>MSSDADAHKVGLIPVTLMVSGNIMGSGVFLLPANLASTGGIAIYGWLVTIIGALGLSMVYAKMSFLDPSPGGSYAYARRCFGPFLGYQTNVLYWLACWIGNIAMVVIGVGYLSYFFPILKDPLVLTITCVVVLWIFVLLNIVGPKMITRVQAVATVLALIPIVGIAVFGWFWFRGETYMAAWNVSGLGTFGAIQSTLNVTLWSFIGVESASVAAGVVKNPKRNVPIATIGGVLIAAVCYVLSTTAIMGMIPNAALRVSASPFGDAARMALGDTAGA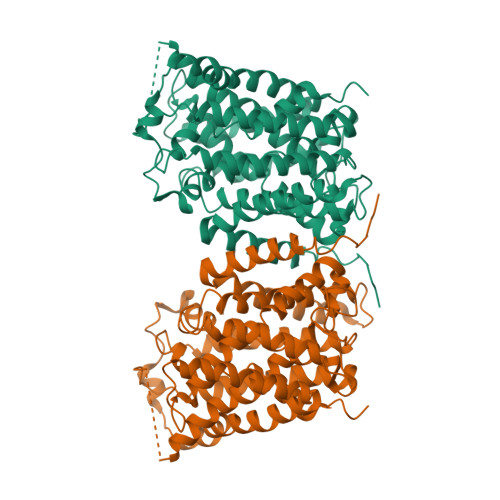IVSFCAAAGCLGSLGGWTLLAGQTAKAAADDGLFPPIFARVNKAGTPVAGLIIVGILMTIFQLSSISPNATKEFGLVSSVSVIFTLVPYLYTCAALLLLGHGHFGKARPAYLAVTTIAFLYCIWAVVGSGAKEVMWSFVTLMVITAMYALNYNRLHKNPYPLDAPISKD[4x]>[4x]MALYGFAQGLIQEAGIRIKQLMEQNLTIETKSNPNDLVTNVDKATEDFIFDTILETYPNHQVLGEEGHGHDIDTSKGTVWVVDPIDGTLNFVHQQENFAISIGIYIDGKPYAGFVYDVMADVLYHAKVGE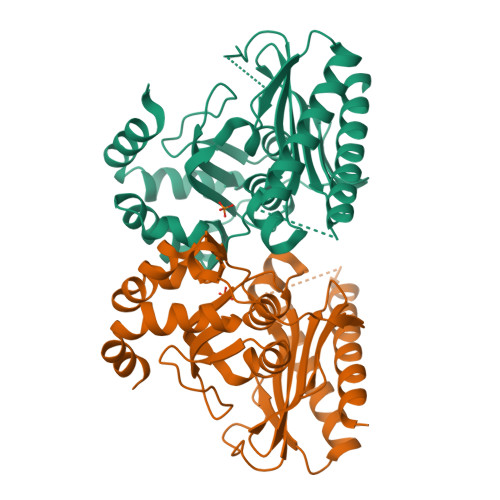GAYRGSQPLKPLNDSNLRQSIIGINPNWLTKPILGEIFKEIVNDSRSARAYGSAALEIVSVATGNLEAYMTPRLQPWDFAGGLVILYEVNGQASNLLGEPLTISGPNSILVGNRGLHQEISNDYLEPHHDALIQLHEQRFKRKSK> MHHHHHHMVHITLDRNTANSWLIISKDRRQVRMGDTHQNVSDNKERFSNYPMVLGAQRFSSGKMYWEVDVTQKEAWDLGVCRDSVQRKGQFSLSPENGFWTIWLWQDSYEAGTSPQTTLHIQVPPCQIGIFVDYEAGVV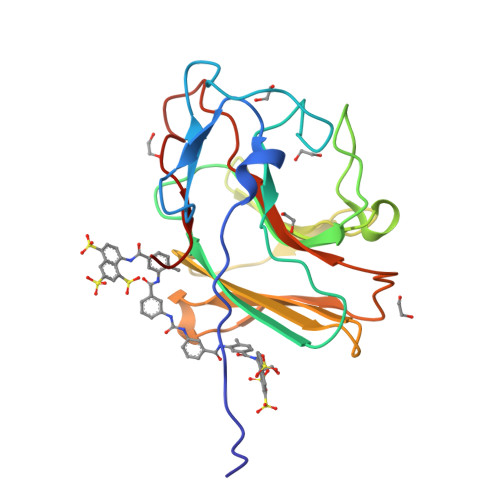SFYNITDHGSLIYTFSECVFAGPLRPFFNVGFNYSGGNAAPLKLCPLKM>[4x]MAEYTLPDLDWDYGALEPHISGQINELHHSKHHATYVKGANDAVAKLEEARAKEDHSAILLNEKNLAFNLAGHVNHTIWWKNLSPNGGDKPTGE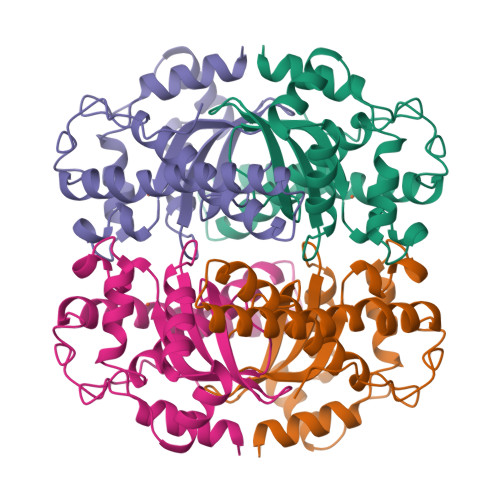LAAAIADAFGSFDKFRAQFHAAATTVQGSGWAALGWDTLGNKLLIFQVYDHQTNFPLGIVPLLLLDMWEHAFYLQYKNVKVDFAKAFWNVVNWADVQSRYAAATSQTKGLIFG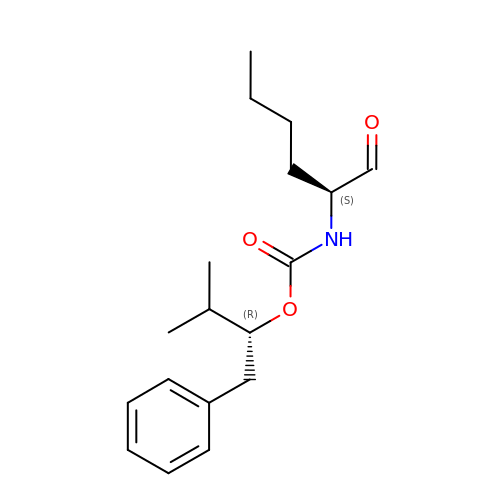(1R)-2-METHYL-1-(PHENYLMETHYL)PROPYL[(1S)-1-FORMYLPENTYL]CARBAMATE | C18 H27 N O3 | ZLZXUNHJWVLGTE-DLBZAZTESA-N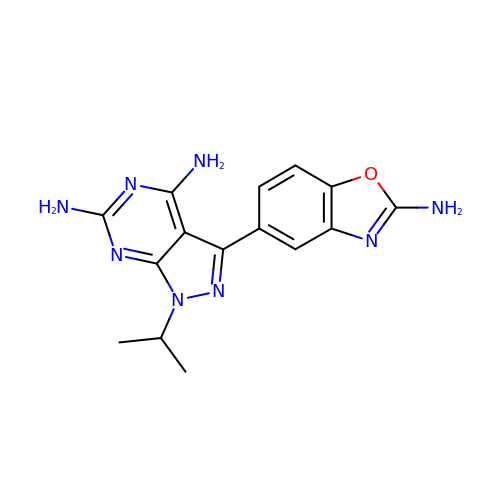3-(2-azanyl-1,3-benzoxazol-5-yl)-1-propan-2-yl-pyrazolo[3,4-d]pyrimidine-4,6-diamine | C15 H16 N8 O | HGZOUPKZPOAOOQ-UHFFFAOYSA-N>AKLTIESTPFNVAEGKEVLLLAHNLPQNRIGYSWYKGERVDGNSLIVGYVIGTQQATPGPAYSGRETIYPNASLLIQNVTQNDTGFYTLQVI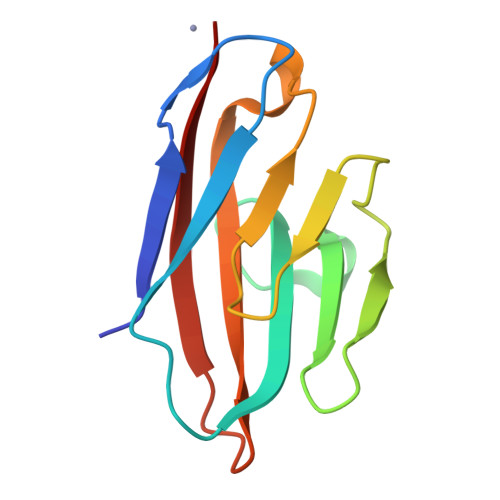KSDLVNEEATGQFHVY[2x]> MLLHLIYGPTCSGKTDMAIQIAQETGWP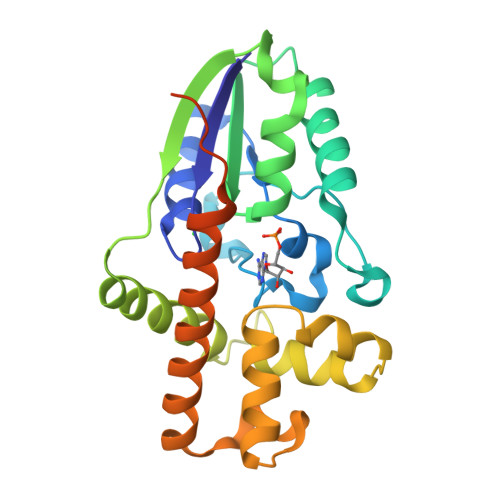VVALDRVQCCPQIATGSGRPLESELQSTRRIYLDSRPLTEGILDAESAHRRLIFEVDWRKSEEGLILEGGSISLLNCMAKSPFWRSGFQWHVKRLRLGDSDAFLTRAKQRVAEMFAIREDRPSLLEELAELWNYPAARPILEDIDGYRCAIRFARKHDLAISQLPNIDAGRHVELIEAIANEYLEHALSQERDFPQWPEDGAGQPVCPVTLTRIRGSRSHHHHHH> XNRVFAEYPDHIQDYFKQSFPKGYSWERSLTFEDGGICIARNDITMEGDTFYNKVRFHGVNFPANGPVMQKKTLKWEPSTEKMYVRDGVLTGDITMALLLEGNAHYRCDSRTTYKAKEKGVKLPGYHLVDHCIEILSHDKDY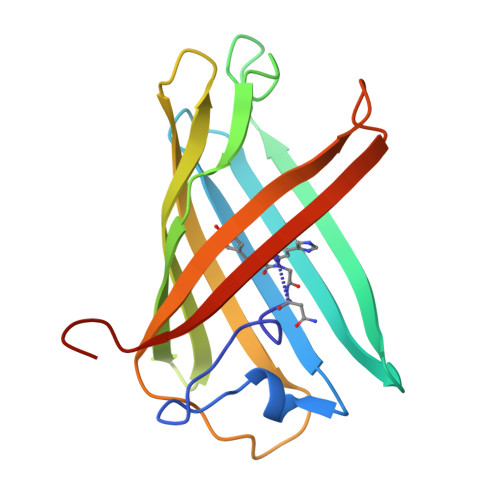NKVKLYEHAVAHSGLPDNARR> MPVEKDLKTAYKALYDEKEPLKALHLYDEILKGSPTNLTALIFKAACLEKLYFGFSDWHSDATMENAKELLDKALMTAEGRGDRSKIGLVNFRYFVHFFNIKDYELAQSYFKKAKNLGYVDDTLPLWEDRLETKLNKKNKKQKDSTNK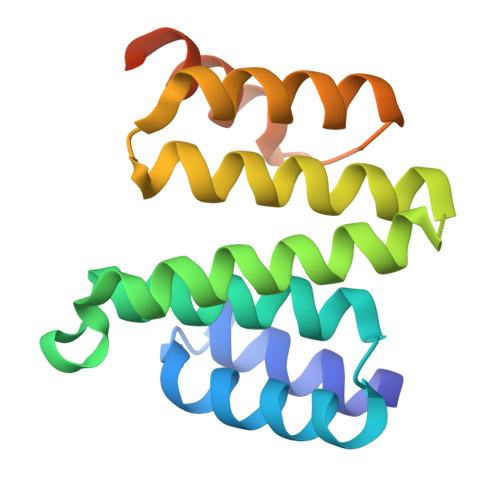HT>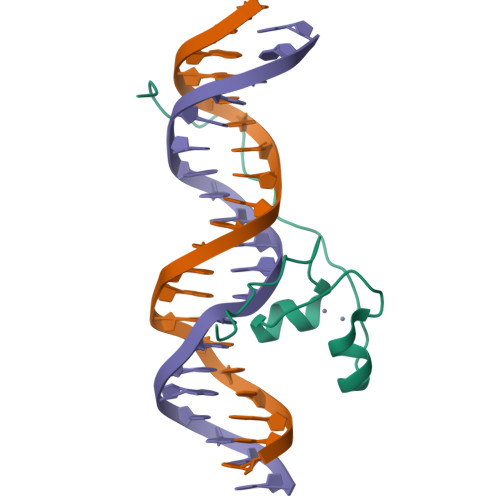 SGKVKKRLPQAKRACAKCQKDNKKCDDARPCQRCIKAKTDCIDLPRKKRPTGVRRGPYK>MKKEVCSVAFLKAVFAEFLATLIFVFFGLGSALKWPSALPTILQIALAFGLAIGTLAQALGPVSGGHINPAITLALLVGNQISLLRAFFYVAAQLVGAIAGAGILYGVAPLNARGNLAVNALNNNTTQGQAMVVELILTFQLALCIFASTDSRRTEPVGSPALSIGLSVTLGHLVGIYFTGCSMNPARSFGPAVVMNRFSPAHWVFWVGPIVGAVLAAILYFYLLFPNSLSL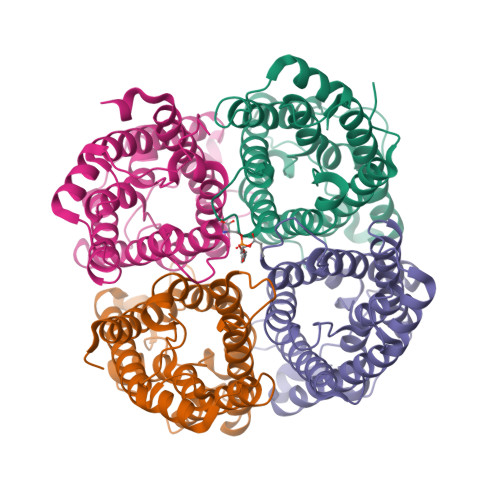SERVAIIKGTYEPDEDWEEQREERKKTMELTTR[4x]> MIPVTELRYFADTQPAYRILKPWWDVFTDYISIVMLMIAVFGGTLQVTQDKMICLPCKWVTKDSCNDSFRGWAAPGPEPTYPNSTILPTPDTGPTGIKYDLDRHQYNYVDAVCYENRLHWFAKYFPYLVLLHTLIFLACSNFWFKFPRTSSKLEHFVSILLKCFDSPWTTRALSETVVEESDPKPAFSKMNGSMDKKSSTVSEDVEATVPMLQRTKSRIEQGIVDRSETGVLDKKEGEQAKALFEKVKKFRTHVEEGDIVYRLYMRQTIIKVIKFILIICYTVYYVHNIKFDVDCTVDIESLTGYRTYRCAHPLATLFKILASFYISLVIFYGLICMYTLWWMLRRSLKKYSFESIREESSYSDIPDVKNDFAFMLHLIDQYDPLYSKRFAVFLSEVSENKLRQLNLNNEWTLDKLRQRLTKNAQDKLELHLFMLSGIPDTVFDLVELEVLKLELIPDVTIPPSIAQLTGLKELWLYHTAAKIEAPALAFLRENLRALHIKFTDIKEIPLWIYSLKTLEELHLTGNLSAENNRYIVIDGLRELKRLKVLRLKSNLSKLPQVVTDVGVHLQKLSINNEGTKLIVLNSLKKMANLTELELIRCDLERIPHSIFSLHNLQEIDLKDNNLKTIEEIISFQHLHRLTCLKLWYNHIAYIPIQIGNLTNLERLYLNRNKIEKIPTQLFYCRKLRYLDLSHNNLTFLPADIGLLQNLQNLAITANRIETLPPELFQCRKLRALHLGNNVLQSLP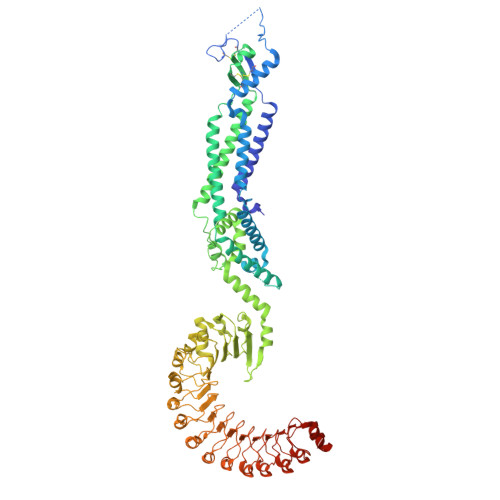SRVGELTNLTQIELRGNRLECLPVELGECPLLKRSGLVVEEDLFNTLPPEVKERLWRADKEQATGGLVPR>[2x]ALGVVGVLESYIGSINNITKQSACVAMSKLLTELNSDDIKKLRDNEELNSPKIRVYNTVISYIESNRKNNKQTIHLLKRLPADVLKKTIKNTLDIHKSITINN

The M2–1 transcription antiterminator factor is a basic protein of 194 amino acids that exists as a stable tetramer in solution and is essential for the complete sequential transcription of mRNAs in HRSV. It harbours four distinct regions: an N-terminal zinc-binding domain (ZBD; residues 7–25), an α-helical tetramer­ization domain (TD; residues 32–49), an RNA-binding core domain (RBD; residues 69–172) and a C-terminal unstructured region (residues 173–194). A crystal structure of the tetrameric M2–1 assembly and an NMR structure of the monomeric M2–1 RBD (residues 58–177; Blondot et al., 2012) have been determined. M2–1 oligomerization is primarily driven by a central tetramerization α-helix and is also stabilized by contacts between the zinc-binding domain and the core of an adjacent monomer. Given the relevance and uniqueness of this viral transcription antiterminator, we set out to investigate its RNA-binding domain (residues 73–194) using X-ray crystallography and folding thermodynamics.

The HRSV M2–1 RBD crystallized with two molecules in the asymmetric unit. The structures from both crystal forms are virtually identical in the core region (residues 58–177), with a root-mean-square deviation (r.m.s.d. on Cα atoms) of 0.3 Å. The elution profile from size-exclusion chromatography indicates that the HRSV M2–1 RBD exists as a monomer in solution. The RNA-binding core domain appears to be a compact and cooperative folding unit in the crystal structure reported here and the previous NMR structure of a similar fragment. The folding studies reveal that although the RBD shows inter-monomer contacts and contacts the ZBD from neighbouring monomers in the tetramer, these do not influence its structure or stability.Here, we employ a bidirectional F420‐reducing [NiFe] hydrogenase from the archaeon Methanosarcina barkeri MS (MbFRH) as a unique model system to yield structural and spectroscopic insights into a scarcely explored reaction intermediate that is the initial target for H2 binding to the active site of the enzyme. Each asymmetric unit contains three subunits, FRH‐A, FRH‐B, and FRH‐G, and a total of four [4Fe4S] clusters as well as a flavin adenine dinucleotide (FAD) cofactor and the [NiFe] active site (detailed below). The FAD and the heterobimetallic [NiFe] center enable the redox conversion of the two substrates, coenzyme F420 and H2, respectively, while the [4Fe4S] clusters mediate intramolecular electron transfer (ET) between the two reaction sites. These features are shared with the related [NiFe] hydrogenase from Methanothermobacter marburgensis (Mm), and both enzymes exhibit a dodecameric overall architecture in a spherical shape.2 Compared to the latter enzyme, however, MbFRH contains two additional cofactors that are both ET‐accessible and solvent‐exposed: a [2Fe2S] cluster bridging two FRH‐G subunits and a mononuclear Fe site in FRH‐A.

While the presence or absence of bridging oxygen ligands can be clearly established from crystal‐structure analyses, H2‐derived (hydride) ligands are only observable in sub‐atomic‐resolution structures, and available crystal structures lacking detectable bridging ligands most likely represent hydride species.9e, 13 Since crystals of MbFRH have been prepared in a mildly reducing atmosphere containing up to 5 % H2, the derived structural data could reflect Nia‐S or a hydride species. IR spectra of MbFRH crystals reveal CO and CN stretching bands at 1945 and 2065/2080 cm−1, respectively, which resemble the IR fingerprint of the Nia‐S state of several [NiFe] hydrogenases.6a In particular, these vibrational frequencies are close to those observed for the as‐isolated regulatory hydrogenase from Ralstonia eutropha (ReRH), which is a spectroscopically valuable yet structurally unexplored reference system for the Nia‐S state. Specifically, a peculiar seesaw‐shaped geometry with trans S−Ni−S angles approaching 120° and 180° was postulated to be mandatory for thermodynamically favorable binding of H2 to Nia‐S.16 In line with this proposal, the [NiFe] active site of MbFRH exhibits trans S−Ni−S angles of 107° and 171°, thereby structurally confirming this unusual geometry of the Nia‐S state. Notably, four‐coordinate NiII sites, as found in Nia‐S, typically exhibit (distorted) square‐planar or tetrahedral coordination geometries. This indicates that the atypical seesaw geometry of this [NiFe] intermediate is dictated by the four‐cysteinate coordination pattern and the protein matrix of [NiFe] hydrogenases.

> TKVVEISPTTRLEGHSKLTLKVNDQGIVERGDWLSITPVRGIEKLAIGKTMEQVPKIASRVCGICPIAHTLASTEAMEASIGCEIPTDAKLLRIILHAANRIHSHALHNILILPDFYIPGTEKKFNLFANEQPARSVMARIVRIREIAQTIAAIAGGEAIHPSNPRIGGMYHNVSPRAKQKMADLAKECLVLVHEQMEFMLDVIRNMQNREFVEVGGKQIPLPKKLGYHNQGVMATAPMYGSSSLDDNPTWDFTRWKETRPWDWYMGEVTIDLEDPSYPIGGTTKVGTKANPQMESCTGVPTYDGQPVEVGPRARLATFKNFDEKGTFAQHIARQMEYPDCCYTILNCLDNLNTSGKVLADHIPQGDGSMGWAANEAPRGSNIHLARVKDGKVRWYDMLVPTTWNFPTCSRALTGAPWQIAEMVVRAYDPCVSCATH;> MIEDPYLGKYVTCVSARSTDKEILKKAQDGGIATALMVYALEEGFIDGTIVAGEGDKPWQPKPVVAMTREDILKARGTRYNISPQISWLKEATRSFGLDKVGVTGVCCQMQAVRKAQLYPINMRDVPGKVAFTVGLFCMENFSYKSLQSIVEDHANQSLGSVKKMEITKGKFWVYTERGNVATVPLKATHKYEQPGCHVCLDYVSNLADISTGSVGSPDGWSTVFIRTKVGNEIWSKAVADGMFETKPIEEVKPGLDLLRKLAKQKIDKNQKTVEERKTFGINKGLRNPYA;> TNKIKIGHVHMSGCTGCLVSLADNNLGLIKILDDYADLVYCLTLADVRHIPEMDVALVEGSVCLQDHESVEDIKETRKKSKIVVALGSCACYGNITRFSRGGQHNQPQHESYLPIGDLIDVDVYIPGCPPSPELIRNVAVMAYLLLEGNEEQKELAGKYLKPLMDLAKRGTSGCFCDLMYDVINQGLCMGCGTCAASCPVHAITLEFGKPQGERDLCIKCGSCYGACPRSFFNLDVISEFENISEIIAKALKD>MHPGEIPRFTQEEYRPPPVSELAAKGTMVGLISAAAINQSIVYSIVSGNEEDKFGINNITGVIYVNAPLDYETRTSYVLRVQADSLEVVLANLRVPSKSNTAKVYIEIQDENDHPPVFQKKFYIGGVSEDARMFASVLRVKATDKDTGNYSAMAYRLIIPPIKEGKEGFVVETYTGLIKTAMLFHNMRRSYFKFQVIATDDYGKGLSGKADVLVSVVNQLDMQVIVSNVPPTLVEKKIEDLTEILDRYVQEQIPGAKVVVESIGARRHGDAFSLEDYTKCDLTVYAIDPQTNRAVDRNELFKFLDGKLLDINKDFQPYYGEGGRILEIRTPEAVTSIKKRGESLGYTE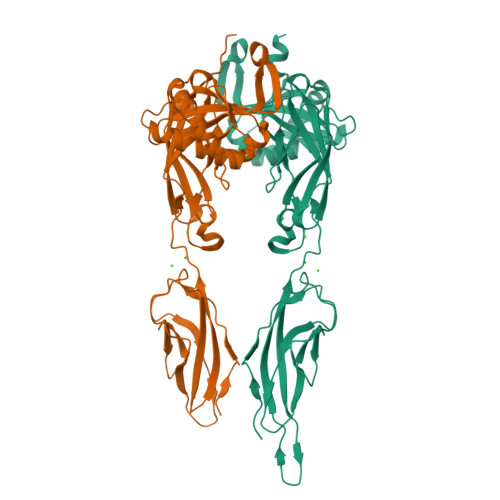LEHHHHHH[2x]> HHHHHHARSVRHIAIPAHRGLITDRNGEPLAVSTPVTTLWANPKELMTAKERWPQLAAALGQDTKLFADRIEQNAEREFIYLVRGLTPEQGEGVIALKVPGVYSIEEFRRFYPAGEVVAHAVGFTDVDDRGREGIELAFDEWLAGVPGKRQVLKDRRGRVIKDVQVTKNAKPGKTLALSIDLRLQYLAHRELRNALLENGAKAGSLVIMDVKTGEILAMTNQPTYNPNNRRNLQPAAMRNRAMIDVFE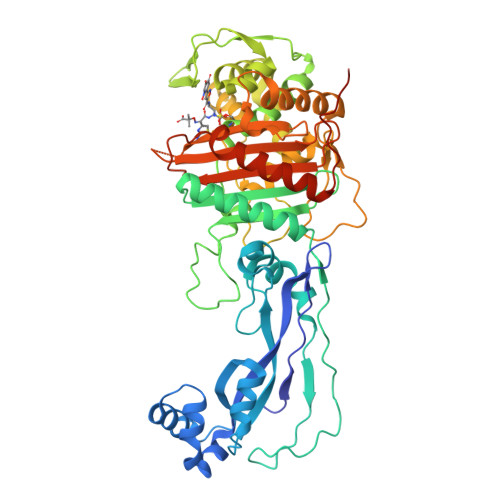PGSTVKPFSMSAALASGRWKPSDIVDVYPGTLQIGRYTIRDVSRNSRQLDLTGILIKSSNVGISKIAFDIGAESIYSVMQQVGLGQDTGLGFPGERVGNLPNHRKWPKAETATLAYGYGLSVTAIQLAHAYAALANDGKSVPLSMTRVDRVPDGVQVISPEVASTVQGMLQQVVEAQGGVFRAQVPGYHAAGKSGTARKVSVGTKGYRENAYRSLFAGFAPATDPRIAMVVVIDEPSKAGYFGGLVSAPVFSKVMAGALRLMNVPPDNLPTATEQQQVNAAPAKGGRG> GEKKECWSWESYLEEQKAITAPVSLFQDSQAVTHNKNGFKLGMKLEGIDPQHPSMYFILTVAEVCGYRLRLHFDGYSECHDFWVNANSPDIHPAGWFEKTGHKLQPPKGYKEEEFSWSQYLRSTRAQAAPKHLFVSQSHSPPPLGFQVGMKLEAVDRMNPSLVCVASVTDV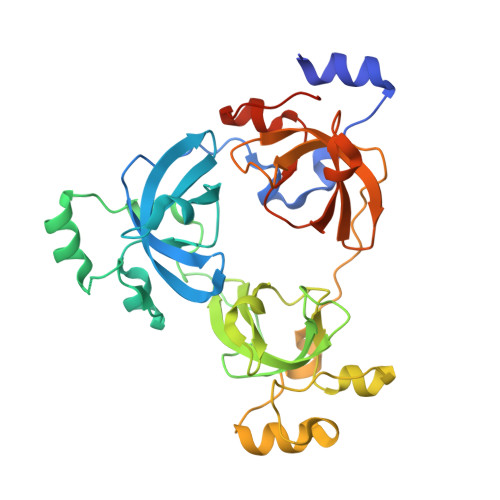VDSRFLVHFDNWDDTYDYWCDPSSPYIHPVGWCQKQGKPLTPPQDYPDPDNFCWEKYLEETGASAVPTWAFKVRPPHSFLVNMKLEAVDRRNPALIRVASVEDVEDHRIKIHFDGWSHGYDFWIDADHPDIHPAGWCSKTGHPLQPPLGPREPSSASPGG>[2x]CGIVGAIAQRDVAEILLEGLRRLEYRGYDSAGLAVVDAEGHMTRLRRLGKVQMLAQAAEEHPLHGGTGIAHTRWATHGEPSEVNAHPHVSEHIVVVHNGIIENHEPLREELKARGYTFVSETDTEVIAHLVNWELKQGGTLREAVLRAIPQLRGAYGTVIMDSRHPDTLLAARSGSPLVIGLGMGENFIASDQLALLPVTRRFIFLEEGDIAEITRRSVNIFDKTGAEVKRQDIESNLQYDAGDKGIYRHYMQKEIYEQPNAIKNTLTGRISHGQVDLSELGPNADELLSKVEHIQILACGTSYNSGMVSRYWFESLAGIPCDVEIASEFRYRKSAVRRNSLMITLSQSGETADTLAGLRLSKELGYLGSLAICNVPGSSLVRESDLALMTNAGTEIGVASTKAFTTQLTVLLMLVAKLSRLKGLDASIEHDIVHGLQALPSRIEQM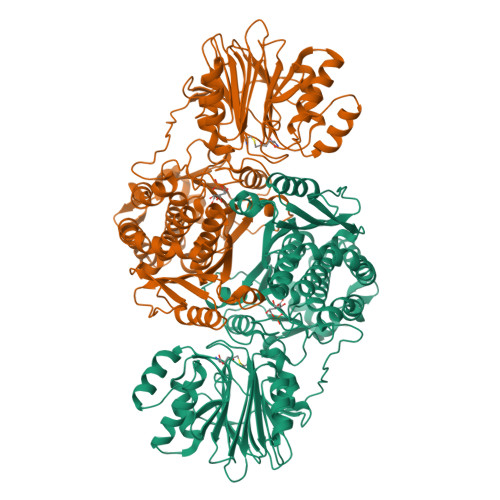LSQDKRIEALAEDFSDKHHALFLGRGDQYPIALEGALKLKEISYIHAEAYAAGELKHGPLALIDADMPVIVVAPNNELLEKLKSNIEEVRARGGQLYVFADQDAGFVSSDNMHIIEMPHVEEVIAPIFYTVPLQLLAYHVALIKGTDVDQPRNLAKSVTVE> GDPIADMIDQTVNNQVNRSLTALQVLPTAANTEASSHRLGTGVVPALQAAETGASSNASDKNLIETRCVLNHHSTQETAIGNFFSRAGLVSIITMPTTGTQNTDGYVNWDIDLMGYAQLRRKCELFTYMRFDAEFTFVVAKPNGELVPQLLQYMYVPPGAPKPTSRDSFAWQTATNPSVFVKMTDPPAQVSVPFMSPASAYQWFYDGYPTFGEHLQANDLDYGQCPNNMMGTFSIRTVGIEKSPHSITLRVYMRIKHVRAWIPRPLRNQPYLFKTNPNYKGNDIKCTSTSRDKITTL;> MGSQVSTQRSGSHENSNSASEGSTINYTTINYYKDAYAASAGRQDMSQDPKKFTDPVMDVIHEMAPPLKSPSAEACGYSDRVAQLTIGNSTITTQEAANIVIAYGEWPEYCPDTDATAVDKPTRPDVSVNRFFTLDTKSWAKDSKGWYWKFPDVLTEVGVFGQNAQFHYLYRSGFCVHVQCNASKFHQGALLVAVLPEYVLGTIAGGTGNENSHPPYATTQPGQVGAVLTHPYVLDAGIPLSQLTVCPHQWINLRTNNCATIIVPYMNTVPFDSALNHCNFGLLVIPVVPLDFNTGATSEIPITVTIAPMCAEFAGLRQAVKQ;> GIPTELKPGTNQFLTTDDGVSAPILPGFHPTPPIHIPGEVHNLLEICRVETILEVNNLKTNETTPMQRLCFPVSVQSKTGELCAAFRADPGRDGPW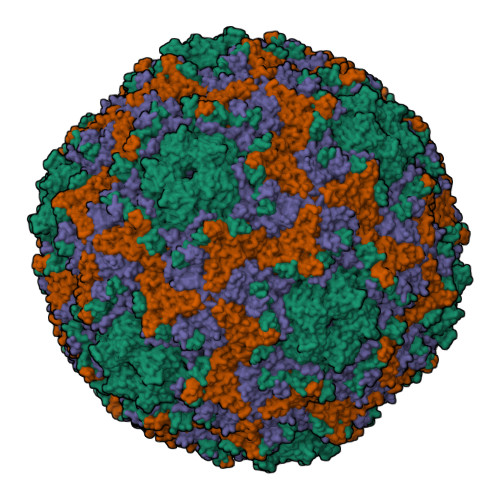QSTILGQLCRYYTQWSGSLEVTFMFAGSFMATGKMLIAYTPPGGNVPADRITAMLGTHVIWDFGLQSSVTLVVPWISNTHYRAHARAGYFDYYTTGIITIWYQTNYVVPIGAPTTAYIVALAAAQDNFTMKLCKDTEDIEQTANIQ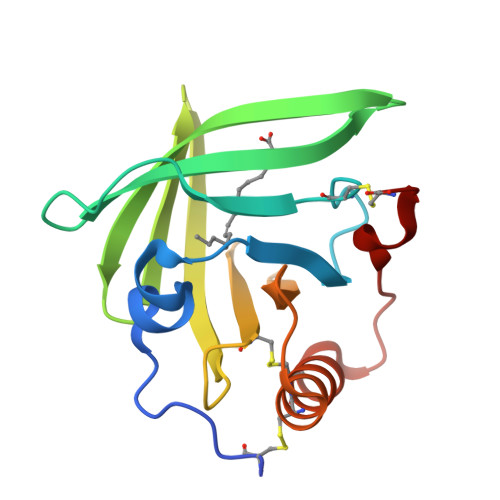> DSESDCTGSEPVDAFQAFSEGKEAYVLVRSTDPKARDCLKGEPAGEKQDNTLPVMMTFKNGTDWASTDWTFTLDGAKVTATLGNLTQNREVVYDSQSHHCHVDKVEKEVPDYEMWMLDAGGLEVEVECCRQKLEELASGRNQMYPHLKDC>MSINLHSAPEYDPSYKLIQLTPELLDIIQDPVQNHQLRFKSLDKDKSEVVLCSHDKTWVLKQRKHSNTVLLMREFVPEQPITFDETLLFGLSKPYMDVVGFAKTESEFETRETHGELNLNSVPIYNGELDFSDKI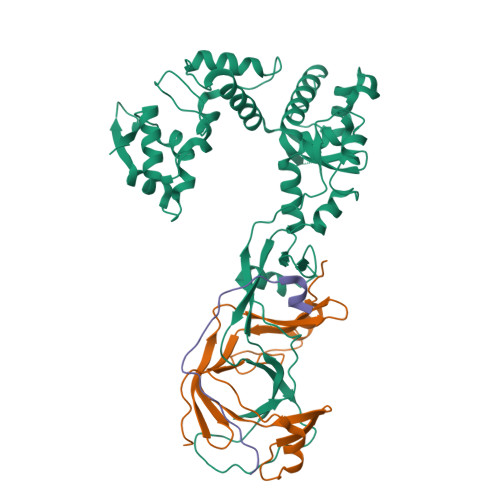MKRSSTKVIGTLEELLENSPCSALEGISKWHKIGGSVKDGVLCILSQDFLFKALHVLLMSAMAESLDLQHLNVEDTHHAVGKDIEDEFNPYTREIIETVLNKFAVQEQEAENNTWRLRIPFIAQWYGIQALRKYVSGISMPIDEFLIKWKSLFPPFFPCDIDIDMLRGYHFKPTDKTVQYIAKSTLPMDPKERFKVLFRLQSQWDLEDIKPLIEELNSRGMKIDSFIMKYARRKRLGKKTVVTSR[2x];>[2x]MPSVDIDASQWQKLTQSREKQTTVITPLGMMMLEIQGELELPKDFASLARRDSPNEGRFSEQDGETLIRFGSLQIDGERATLFVGKKQRLLGKVTKLDVPMGIMHFNSKDNKVELVDVMKYKVIFKDRPLPIM;>SGKVKTGLNSSSSTIDFFKNQYGLLKQTQELEETQKTIGSDETNQADDCNQTVKIWVKYNEGFSNAVRKNVTWNNLWE[2x]4-{hydroxy[(phosphonooxy)acetyl]amino}butyl dihydrogen phosphate | 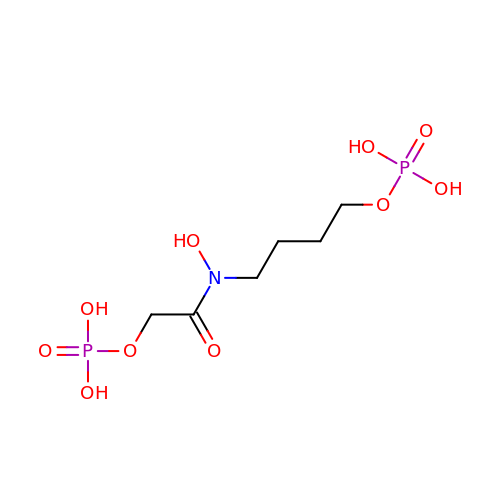C6 H15 N O10 P2 | GZQWGEFAYHQQKX-UHFFFAOYSA-N>GKNEIAQSGEDFKSFLDKFTSSAAFQY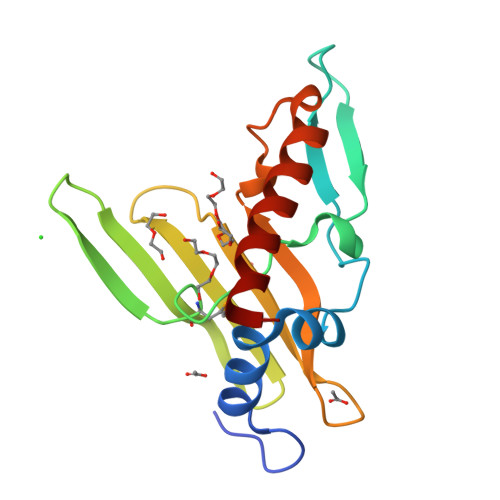TRIKFPLKTPITLLADDGETEKTFPFTKEKWPLLDSETMKEERIEQEEGGIYVSKFTLNEPVHKVFEAGYEESEIDLRVEFEQAADGKWYVVDCYTGWYGYDLPIGELKQTIQQVKEENAAFKEIHP[4x]> QFAKPEDAVKYRQSALTLMASHFGRMTPVVKGQAPYDAAQIKANVEVLKTLSALPWAAFGPGTEGGDARPEIWSDAASFKQKQQAFQDNIVKLSAAAD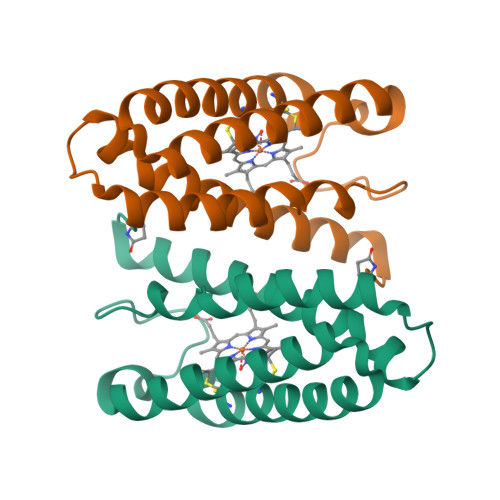AGDLDKLRAAFGDVGASCKACHIAYRKKK>SVDHGFLVTRHSQTIDDPQCPSGTKILYHGYSLLYVQGNERAHGQDLGTAGSCLRKFSTMPFLFCNINNVCNFASRNDYSYWLSTPEPMPMSMAPITGENIRPFISRCAVCEAPAMVMAVHSQTIQIPPCPSGWSSLWIGYSFVMHTSAGAEGSGQALASPGSCLEEFRSAPFIECHGRGTCNYYANAYSFWLATIERSEMFKKPTPSTLKAGELRTHVSRCQVCMRRT[4x];>[2x]SVSIGYLLVKHSQTDQEPMCPVGMNKLWSGYSLLYFEGQEKAHNQDLGLAGSCLARFSTMPFLYCNPGDVCYYASRNDKSYWLSTTAPLPMMPVAEDEIKPYISRCSVCEAPAIAIAVHSQDVSIPHCPAGWRSLWIGYSFLMHTAAGDEGGGQSLVSPGSCLEDFRATPFIECNGGRGTCHYYANKYSFWLTTIPEQSFQGSPSADTLKAGLIRTHISRCQVCMKNL

Basement membranes are extracellular structures of epithelia and endothelia that have collagen IV scaffolds of triple α-chain helical protomers that associate end-to-end, forming networks. At the C-termini, interactions occur between the trimeric NC1 domains of two protomers, forming a hexamer of these domains reinforced by sulfilimine cross-links. Recent studies in one of our laboratories revealed that the NC1 domains function as recognition modules, directing the selection and assembly of α-chains into protomers and networks.

We validated the use of self-assembled recombinant NC1 domains to reflect natural structures by generating the same α121NC1 hexamer as previously isolated from BMs from a 2:1 mixture of pure α1NC1 and α2NC1 chains. Crystals of recombinant α121NC1 diffracted X-rays to 2.8 Å resolution and had the same architecture and folding as the α121NC1 hexamer isolated from BMs (the r.m.s.d. for the superimposition of all Cα atoms of the hexamer is 0.48 Å). The recombinant α121NC1 hexamer was composed of two identical protomers formed by two α1NC1 domains and one α2NC1 domain. Each individual chain (designated α1NC1α121 and α2NC1α121) had an identical fold and relations to its natural counterpart (Than et al., 2002; Sundaramoorthy et al., 2002; Vanacore et al., 2004). Thus, recombinant NC1 chains seem to be appropriate for the formation and structural characterization of collagen IV NC1-domain assemblies. Therefore, the covalent modifications and/or cross-links found in natural α121NC1 hexamers or potential directive roles of the collagenous domains or other macromolecular components do not seem to be essential for the correct self-assembly of α121NC1. In fact, we show here that 2:1 mixtures of α1NC1 and α2NC1 chains spontaneously generate the natural α121NC1 heterohexamer. Spontaneous assembly has been proposed for α121NC1, where the α2NC1 chain shows a higher affinity to interact with α1NC1 than with itself.> MANELTWHDVLAEEKQQPYFLNTLQTVASERQSGVTIYPPQKDVFNAFRFTELGDVKVVILGQDPYHGPGQAHGLAFSVRPGIAIPPSLLNMYKELENTIPGFTRPNHGYLESWARQGVLLLNTVLTVRAGQAHSHASLGWET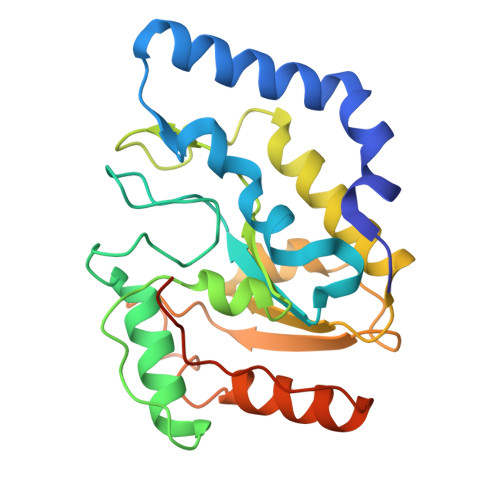FTDKVISLINQHREGVVFLLWGSHAQKKGAIIDKQRHHVLKAPHPSPLSAHRGFFGCNHFVLANQWLEQRGETPIDWMPVLPAESELEHHHHHH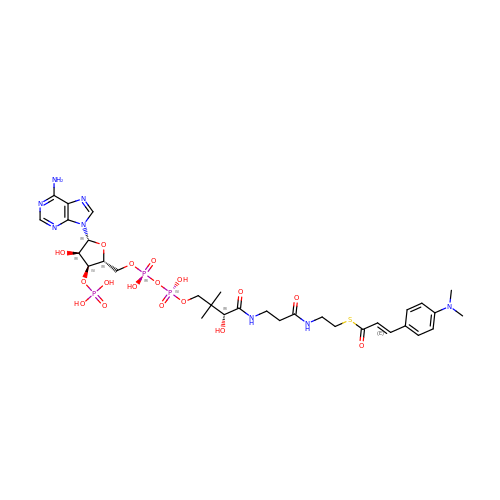4-(N,N-DIMETHYLAMINO)CINNAMOYL-COA | C32 H47 N8 O17 P3 S | WWUPGKDRUIPTRA-XITLLWRLSA-N>GAMGGMHLVGVLDIAKDILKANKRLADKNRKLLNKHGVVAFDFMGAIGSGKTLLIEKLIDNLKDKYKIACIAGDVIAKFDAERMEKHGAKVVPLNTGKECHLDAHLVGHALEDLNLDEIDLLFIENVGNLICP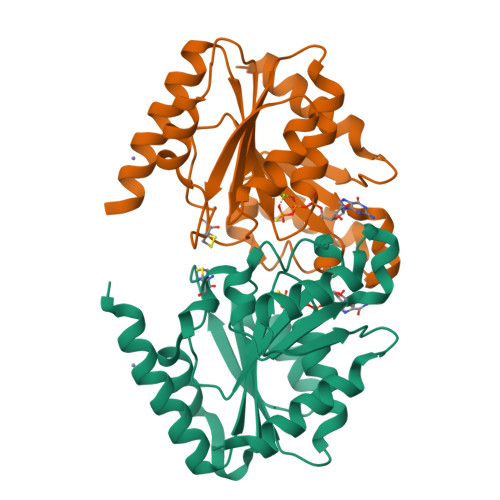ADFDLGTHKRIVVISTTEGDDTIEKHPGIMKTADLIVINKIDLADAVGADIKKMENDAKRINPDAEVVLLSLKTMEGFDKVLEFIEKSVKEVK[2x]Target-based azole resistance in Candida albicans involves overexpression of the ERG11 gene encoding lanosterol 14α-demethylase (LDM), and/or the presence of single or multiple mutations in this enzyme. The azole antifungals inhibit sterol 14α-demethylase (CYP51, SDM), thereby preventing biosynthesis of the essential and fungal specific sterol ergosterol, and resulting in the collateral synthesis of toxic sterols. We have used, as surrogates, structurally aligned mutations in recombinant hexahistidine-tagged full-length Saccharomyces cerevisiae LDM6×His (ScLDM6×His) to elucidate how differential susceptibility to azole drugs is conferred by LDM of the C. albicans Darlington strain. Phenotypes and high-resolution X-ray crystal structures were determined for the surrogate enzymes in complex with representative short-tailed (voriconazole) and long-tailed (itraconazole) triazoles.

The ScLDM6×His Y140H I471T mutant provides a surrogate X-ray crystal structure for the clinically relevant Darlington LDM mutant of C. albicans, and for the LDM Y131F I475T mutant from the phytopathogen P. pachyrhizi. Similar crystals of ScErg11p6×His Y140H I471T in complex with VCZ formed after 20 days of incubation under a single experimental condition (46% PEG 400 pH 9.2). The VCZ in the double mutant showed the same configuration as in ScLDM6×His or ScLDM6×His I471T in complex with VCZ, but was slightly displaced towards H140 and more towards helix I (by ~0.7 Å) than in ScLDM6×His Y140H. The structure of ScLDM6×His Y140H I471T in complex with the VCZ structure also included a single water molecule, 3.6 Å from the tertiary alcohol of VCZ, that formed hydrogen bonds with the heme ring C propionate and a nitrogen of the histidine imidazole ring, but not VCZ. In contrast, both ScLDM6×His Y140H and ScLDM6×His Y140H I471T in complex with VCZ have no AO, but have an open SEC of a similar cross-sectional area at its narrowest point, i.e., the opening bounded by the M509 methyl and H381 imidazole nitrogen, and the F241 benzene ring and T511 sidechain methyl is ~48 Å2 for ScLDM6×His Y140H in complex with VCZ, and ~49 Å2 for ScLDM6×His Y140H I471T in complex with VCZ. The lower resolution (2.9 Å) of the ScLDM6×His Y140H + I471T structure may have limited the observation of discrete structural changes, such as the location of key water molecules. In contrast, it was not apparent how the Y140H and I471T mutations interact to confer preferential high-level resistance to the short-tailed azole VCZ, which appears to bind in the active site in comparable conformations in the Y140H and Y140H I471T enzymes. Unfortunately, the structures obtained do not elucidate how the Y140H and I471T mutations interact to confer enhanced resistance to short-tailed azoles, i.e., the double mutation maintains enzyme function in the presence of the short-tailed triazole inhibitors FLC and VCZ.

> MSATKSIVGEALEYVNIGLSHFLALPLAQRISLIIIIPFIYNIVWQLLYSLRKDRPPLVFYWIPWVGSAVVYGMKPYEFFEECQKKYGDIFSFVLLGRVMTVYLGPKGHEFVFNAKLADVSAEAAYAHLTTPVFGKGVIHDCPNSRLMEQKKFVKGALTKEAFKSYVPLIAEEVYKYFRDSKNFRLNERTTGTIDVMVTQPEMTIFTASRSLLGKEMRAKLDTDFAYLYSDLDKGFTPINFVFPNLPLEHYRKRDHAQKAISGTYMSLIKERRKNNDIQDRDLIDSLMKNSTYKDGVKMTDQEIANLLIGVLMGGQHTSAATSAWILLHLAERPDVQQELYEEQMRVLDGGKKELTYDLLQEMPLLNQTIKETLRMHHPLHSLFRKVMKDMHVPNTSYVIPAGYHVLVSPGYTHLRDEYFPNAHQFNIHRWNNDSASSYSVGEEVDYGFGAISKGVSSPYLPFGGGRHRCTGEHFAYCQLGVLMSIFIRTLKWHYPEGKTVPPPDFTSMVTLPTGPAKIIWEKRNPEQKIGGRHHHHHH>[2x]MVRKVLMICLGNICRSPIAEVVMVDTLEKANVKDVEVDSAAIGGWHVGNRAD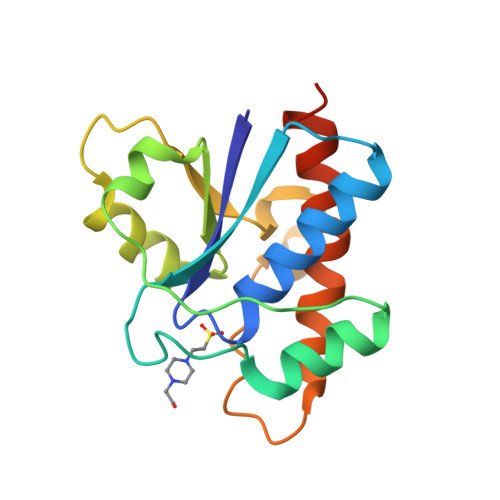PRAISTLQKHGLKCTHIVRQIRKQDFSEFDYIFGMDEDNMSELRRLAPKGSKAELLMLGDFGLEKKNRIIEDPYYERGAEGFETAYQQCVVACAAFMKERLQKLEHHHHHH>INMEEIREFAKNFKIRRLSLGLTQTQVGQAMTATEGPAYSQSAISRFEKLDITPKSAQKLKPVLEKWLNEAELRNQEGQQNLMEFVGGEPSKKRKRRTSFTPQAIEALNAYFEKNPLPTGQEITEMAKELNYDREVVRVWFSN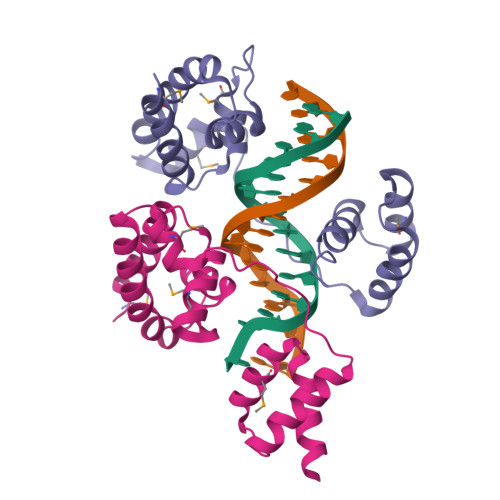RRQTLKNT[8x]> MASMKKKGSVVIVGRINLSGDTAYAQQTRGEEGCQETSQTGRDKNQVEGEVQIVSTATQTFLATSINGVLWTVYHGAGTRTIASPKGPVTQMYTNVDKDLVGWQAPQGSRSLTPCTCGSSDLYLVTRHADVIPVRRRGDSRGSLLSPRPISYLKGSAGGPLLCPAGHAVGIFKAAVSTRGVAKAVDFIPVESLETTMR

The HCV NS3/4A protease – a chymotrypsin-like serine protease – is a prime therapeutic target that cleaves four known sites along the virally encoded polyprotein. The NS3/4A protease also hydrolyzes two human proteins, TRIF and MAVS, which are part of the innate immune system, thereby confounding the innate immune response to viral infection. In this study, we report that four chemically representative protease inhibitors – telaprevir, danoprevir, vaniprevir and MK-5172 – exhibit distinct susceptibilities to the protease variants R155K, A156T and D168A. To elucidate the underlying mechanism by which chemically diverse inhibitors bind to the wild-type protease and drug-resistant variants, crystal structures were determined for 16 inhibitor-protease complexes. These complexes include wild-type protease and resistant variants R155K, D168A and A156T each bound to telaprevir, danoprevir, vaniprevir and MK-5172, with resolutions ranging from 1.10–2.50 Å; S139A protease variants were used except for telaprevir, which requires covalent bond formation with the serine 139 for efficient binding.

Relative to the wild type, R155K caused large reductions in potency for danoprevir and vaniprevir, but MK-5172 remained highly active (R155K IC50 = 0.55 nM). For both danoprevir and vaniprevir, the R155K mutation disrupted the favorable cation-π stacking interactions with the P2 isoindoline moieties, causing significant reductions in drug potencies. In danoprevir, the P2 isoindoline moiety shifted in response to R155K and D168A mutations, making extensive interactions with the catalytic D81. Danoprevir's isoindoline moiety bound in two conformations in the wild-type complex, but adopted a single conformation in mutant complexes. R155K and D168A mutations confer danoprevir and vaniprevir resistance by disrupting favorable cation-π stacking interactions with R155.>[3x]HHHHHHGGCPSQCSCRGTYVDCDSRRLASVPAGIPTNVQILNLYNNQITNLEPGVFDRLVNLQKLYLSGNQLQALPVGVFDKLSQLTFLSLDENKLTALPNGVFDKLTELTYLNLNTNQL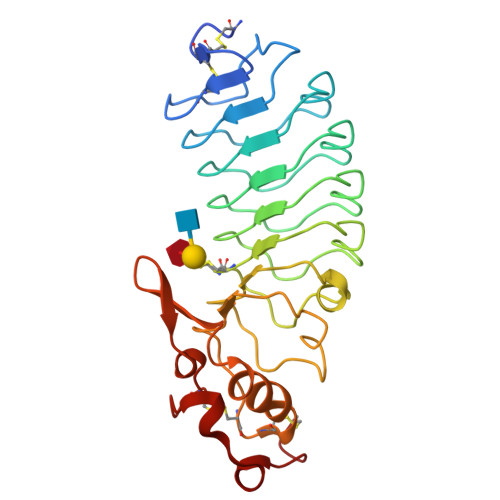TALPEGVFDRLVHLKELLMCCNKLTELPRGIERLTHLTHLALDQNQLKSIPHGAFDRLSSLTHAYLFGNPWDCECRDIMYLRNWVADHTSIVMRWDGKAVNDPDSAKCAGTNTPVRAVTEASTSPSKC>[2x]SCYIYWDKIKRIASRLEGMNYHFDEMDTSGVMPLL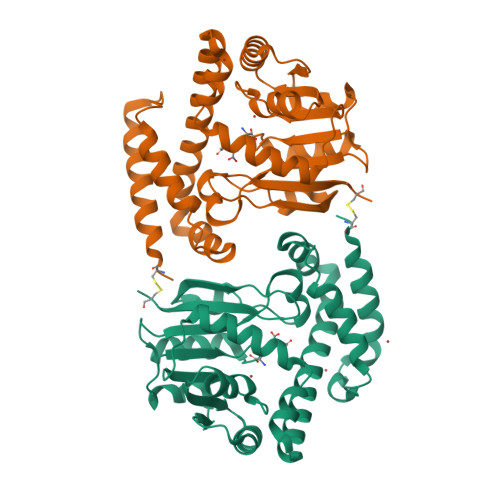DEIEEIAHDSTIDFESAKHILDDAEMNHALSLIRKFYVNLGMKLQMEKAQEVIESDSPWETLRSFYFYPRYLELLKNEAALGRFRRGERAVFIGGGPLPLTGILLSHVYGMRVNVVEIEPDIAELSRKVIEGLGVDGVNVITGDETVIDGLEFDVLMVAALAEPKRRVFRNIHRYVDTETRIIYRTYTGMRAILYAPVSDDDITGFRRAGVVLPSGKVNNTSVLVFKCPKGELNSKLEGKPIPNPLLGLDSTRTGHHHHHH>GLVYPCGACRSEVNDDQDAILCEASCQKWFHRECTGMTESAYGLLTTEASAVWACDLCLKTKEGSGS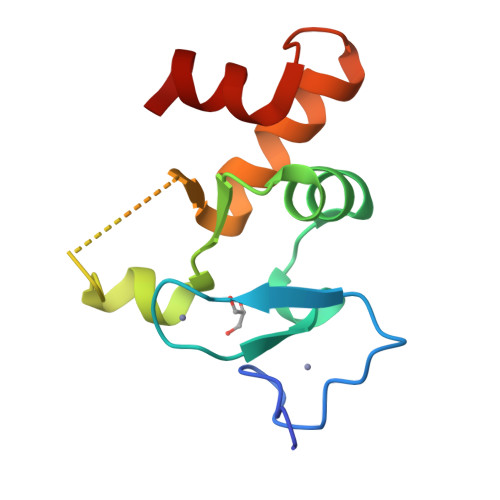GSGSQFVYVFTTHLANTAAEAVLQGRADSILAYHQQNV[2x]(2S)-2-{[2-(L-cysteinylamino)-2-deoxy-alpha-D-glucopyranosyl]oxy}butanedioic acid | C13 H22 N2 O10 S | 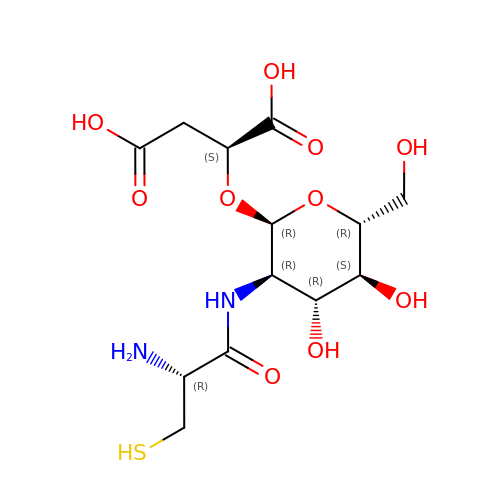UHNHELGKNQMNGF-AOQKXWSCSA-N>[2x]MHII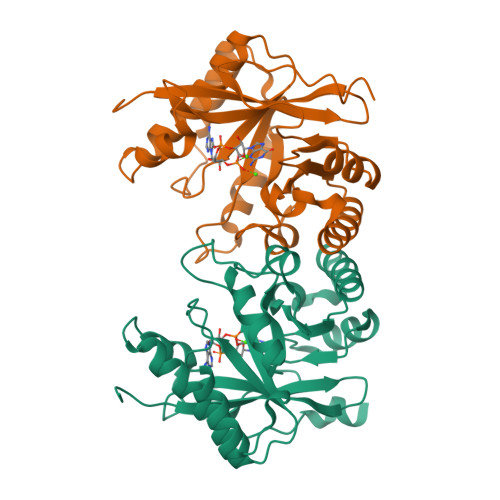PVASDPKTCSSGVNENSLDFDFTMAFQPIVNCRTKEIFGYEALVRGLNNESAYSVISRVNEDNRYLFDQMCRVKAIALAAKLGLTSKLSINFLPNAIYVPERCIRTTLEAAKRYQFPIENIMFEFTEAERVEDVNHIKRIVEYYKSLGFQTAIDDFGSGYSGLNLLADFQTNIVKVDMGLIRNIHADQVRQSIMKNCLKLFSDLNIQPLAEGVESHAEFAWLKAAGVELMQGYYFAKPGFESLPSVNPEFSEA DAIDZIN 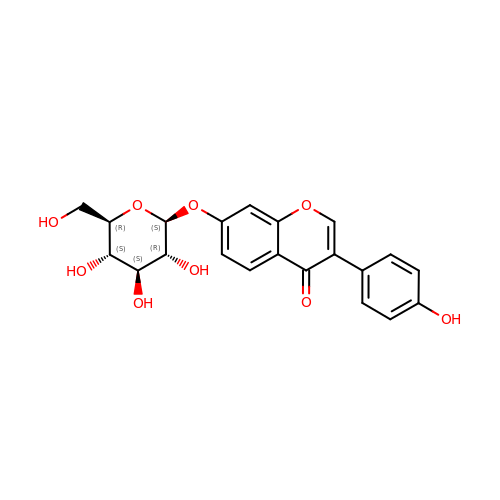| C21 H20 O9 | KYQZWONCHDNPDP-QNDFHXLGSA-N>MVEKEEAGGGISEEEAAQYDRQIRLWGLEAQKRLRASRVLLVGLKGLGAEIAKNLILAGVKGLTMLDHEQVTPEDPGAQFLIRTGSVGRNRAEASLERAQNLNPMVDVKVDTEDIEKKPESFFTQFDAVCLTCCSRDVIVKVDQICHKNSIKFFTGDVFGYHGYTFANLGEHEFVEEKTKVAKVSQGVEDGPDTKRAKLDSSETTMVKKKVVFCPVKEALEVDWSSEKAKAALKRTTSDYFLLQVLLKFRTDKGRDPSSDTYEEDSELLLQIRNDVLDSLGISPDLLPEDFVRYCFSEMAPVCAVVGGILAQEIVKALSQRDPPHNNFFFFDGMKGNGIVECLGPK[2x];>[2x]MALSRGLPRELAEAVAGGRVLVVGAGGIGCELLKNLVLTGFSHIDLIDLDTIDVSNLNRQFLFQKKHVGRSKAQVAKESVLQFYPKANIVAYHDSIMNPDYNVEFFRQFILVMNALDNRAARNHVNRMCLAADVPLIESGTAGYLGQVTTIKKGVTECYECHPKPTQRTFPGATIRNTPSEPIHCIVWAKYLFNQLFGEEDADQEVSPDRADPEAAWEPTE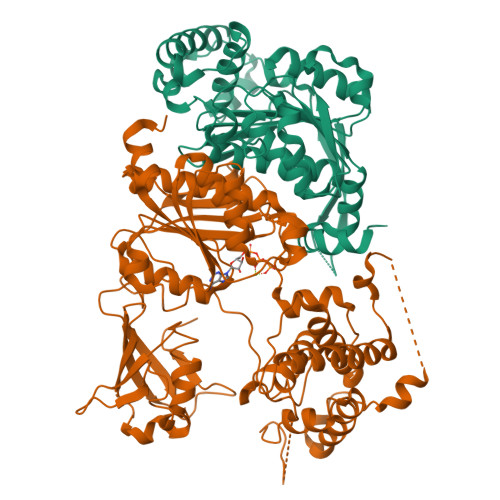AEARARASNEDGDIKRISTKEWAKSTGYDPVKLFTKLFKDDIRYLLTMDKLWRKRKPPVPLDWAEVQSQGEETNASDQQNEPQLGLKDQQVLDVKSYARLFSKSIETLRVHLAEKGDGAELIWDKDDPSAMDFVTSAANLRMHIFSMNMKSRFDIKSMAGNIIPAIATTNAVIAGLIVLEGLKILSGKIDQCRTIFLNKQPNPRKKLLVPCALDPPNPNCYVCASKPEVTVRLNVHKVTVLTLQDKIVKEKFAMVAPDVQIEDGKGTILISSEEGETEANNHKKLSEFGIRNGSRLQADDFLQDYTLLINILHSEDLGKDVEFEVVGDAPEKVGPKQAEDAAKSITNGSDDGAQPSTSTAQEQDDVLIVDSDEEDSSNNADVSEEERSRKRKLDEKENLSAKRSRIEQKEELDDVIALD> GPHMPGDYLIHPEHGVGQYLGLETREVLGVKRDYLVLRYKGEGK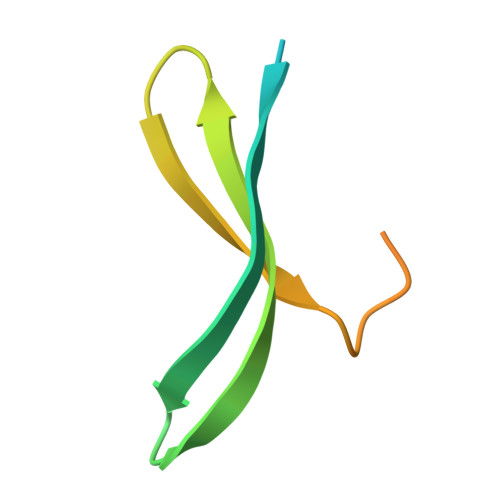LYLPVEQLPLLKRHPGTTDDPPELSSL>[2x]MVLYFIGLGLYDERDITVKGLEIAKKCDYVFAEFYTSLMAGTTLGRIQKLIGKEIRVLSREDVELNFENIVLPLAKENDVAFLTPGDPLVATTHAELRIRAKRAGVESY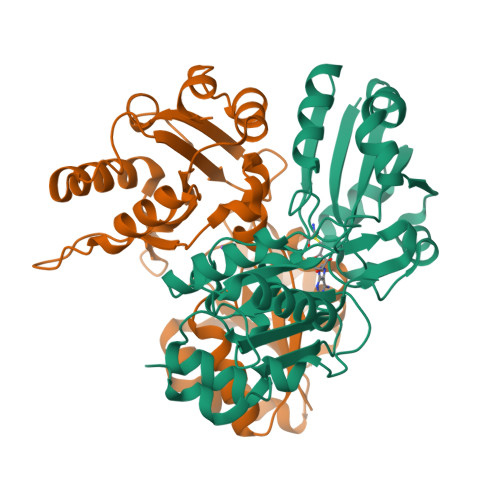VIHAPSIYSAVGITGLHIYKFGKSATVAYPEGNWFPTSYYDVIKENAERGLHTLLFLDIKAEKRMYMTANEAMELLLKVEDMKKGGVFTDDTLVVVLARAGSLNPTIRAGYVKDLIREDFGDPPHILIVPGKLHIVEAEYLMEIAGAPREILRVNV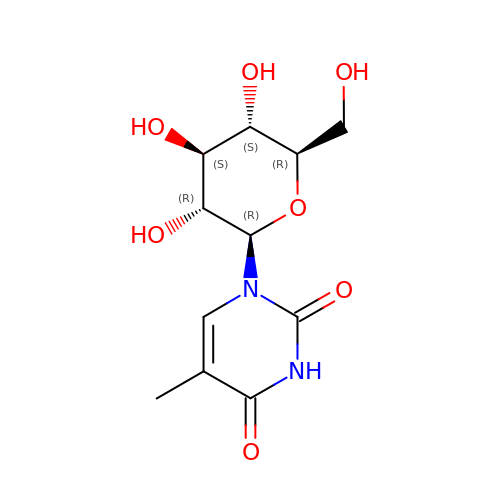1-beta-D-glucopyranosyl-5-methylpyrimidine-2,4(1H,3H)-dione | C11 H16 N2 O7 | RMXUFBPORJBBEZ-HPFNVAMJSA-N Artificially expanded genetic information systems (AEGIS) were developed to expand the diversity and functionality of biological systems. To establish the effectiveness of AEGIS toward nanotechnological applications, we investigated the ability of a six-letter alphabet composed of A:T, G:C and synthetic Z:P (Z, 6-amino-3-(1′-β-d-2′-deoxy ribofuranosyl)-5-nitro-(1H)-pyridin-2-one; P, 2-amino-8-(1′-β-d-2′-deoxyribofuranosyl)-imidazo-[1,2a]-1,3,5-triazin-(8H)-4-one) base pairs to engage in 3D self-assembly. To carry out this investigation, we employed the tensegrity triangle, a reliable DNA motif which self-assembles into 3D crystals with rationally designed symmetry.

In this paper, the six pairing nucleobases were incorporated into the tensegrity triangle motif in order to show that they behave similarly to the natural nucleic acids, exhibiting the conformational diversity to self-assemble into 3D macromolecular objects. This represents the first case where a nonduplex structure has incorporated any component of any artificially expanded genetic information system by Watson–Crick parity. In this study, a “two-turn” tensegrity triangle, possessing 21 bp per edge, was designed with monomer C:G sticky ends and 5′-phosphate attached to the helical strands (green strands). This basic design was modified by adding Z and P at strategic positions within the triangle core, where stability is highest and crystallographic B-factors have been shown to be minimized. Diffraction was obtained to 3.56 Å, and data were processed into the R3 space group, typical of well-constructed tensegrity triangles. Overall, we confirm that the morphology of the crystal is isomorphic to the other two turn tensegrity triangle crystals. We found that, excluding the junctions, the helicity of the 6 bp regions were 9.85 and 9.84 bp/T, for the Z:P and G:C triangles, respectively, while including the junctions yielded helicity values of 10.34 and 10.35 bp/T, respectively. As the Z:P pair in this study is adjacent to the J1 junction, we would expect differences in local geometry to be absorbed and computed by the junction valve. The introduction of AEGIS nucleobases was successful, and the overall result was isomorphic to the four-letter Watson–Crick system. To demonstrate the generality of this result, we moved the position of Z:P base pairs in the DNA tensegrity triangle and found that it had little effect on the formation of DNA motif and crystallization process except placing it on the nick or junction positions.

> GAGCAGCCTXTACGGACATCA;> CCGTAXA;> GGCTGCT;> CTGATGT> MSVLTKAIVNADAEARYLSPGELDRIKSFVASGERRLRIAQTLTEARERIVKQAGDQLFQIRPDVVSPGGNAYGEKMTALCLRDLDYYLRLVTYGIV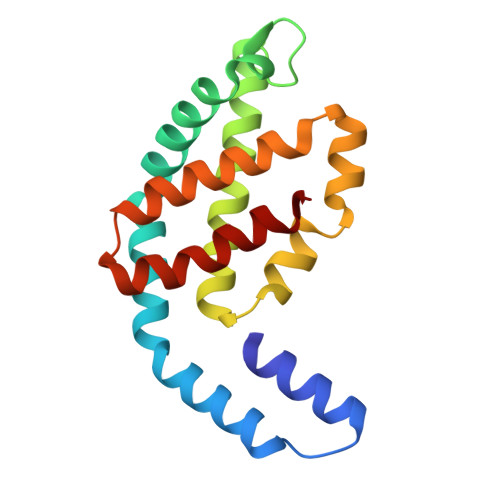AGDVTPIEEIGIIGVKEMYNSLQTPIPAVAEGVRAMKNVATSLLSGDDAAEAGFYFDYLVGAMQ>MEFWGVAVTPKNATKVTPEEDSLVHISQASLDCTVKSGESVVLSVTVGGAKLVIGTLSQDKFPQIS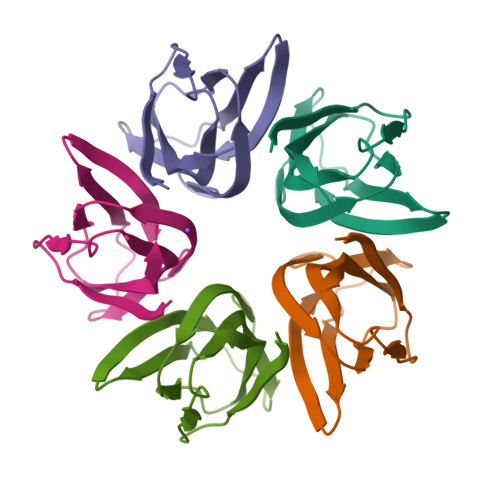FDLVFDKEFELSHSGTKANVHFIGYKSPNL[5x]>MRRLTAALCALTLLSTGAQAQTIKDFLAVAMKKWTAPFEPFQLID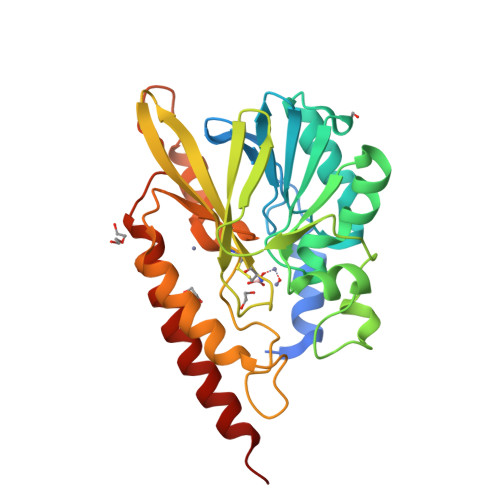NIYYVGTDGIAVYVIKTSQGLILMDTAMPQSTGMIKDNIAKLGFKVADIKLILNTHAHLDHTGGFAEIKKETGAQLVAGERDKPLLEGGYYPGDEKNEDLAFPAVKVDRAVKEGDRVTLGDTTLTAHATPGHSPGCTSWEMTVKDGKEDREVLFFCSGTVALNRLVGQPTYAGIVDDYRATFAKAKAMKIDVLLGPHPEVYGMQAKRAEMKDGAPNPFIKPGELVTYATSLSEDFDKQLAKQTAALEKK[2x]>AEAGITGTWYAQLGDTFIVTAGADGALTGTYEAAVGDDDGDDDGDDDGAESRYVLTGRYDSAPATDGSGTALGWTVAWKNNYRNAHSATTWSGQYVGGAEARINTQWLLTSGTTEANAWKSTLVGHDTFTKVKPSAAS[2x];>AEAGITGTWYNQLGSTFIVTAGADGALTGTYESAVGNAESRYVLTGRYDSAPATDGSGTALGWTVAWKNNYRNAHSATTWSGQYVGGAEARINTQWLLTSGTTEANAWKSTLVGHDTFTKVKPSAAS[2x]

The femtomolar affinity of streptavidin/avidin for biotinylated targets, combined with resilience to harsh conditions and an on-rate of ~ 107 M− 1 s− 1, is the basis for biotin's central role as a specific biological “glue” in diverse research methods and biotechnologies. We previously generated streptavidin heterotetramers with exactly one, two, or three functional biotin-binding sites, through purifying tetramers containing defined numbers of non-biotin-binding “Dead” and His6-tagged wild-type subunits. However, tetramers with two functional and two Dead subunits can assemble in three different arrangements. To generate a controlled and stable bridge for bionanotechnology, we demonstrate here a method for the simple isolation of streptavidin variants with precise cis-divalent or 1,3 trans-divalent arrangements.

In the 1,2 arrangement the biotin-binding sites of streptavidin are in a cis configuration as the binding sites both point in the same direction. To isolate cis-divalent streptavidin (1,2 arrangement of biotin-binding subunits), we introduced a series of aspartates into the loop between β-strands 3 and 4 (L3,4) of the Dead subunit. Introduction of the charges in this position means that in the 1,3 and 1,4 arrangements, these charged regions should be far apart, while in the 1,2 arrangement, the charged loops should be apposed. Since L3,4 is important for biotin binding affinity, it was necessary to insert these residues on the Dead subunit, so that the cis-divalent streptavidin could maintain high biotin binding affinity. Overall, the introduction of a series of negative charges into the surface-exposed 3,4-loop of streptavidin allowed the isolation of a second divalent species, cis-divalent. However, one condition obtained using the Morpheus crystal screen yielded the desired asymmetric unit for the cis-divalent streptavidin containing all four subunits. The obtained 1,3 trans-divalent crystal structure was solved at 1.6 Å resolution, and cis-divalent streptavidin was solved at 1.4 Å resolution, with the phases in each case solved using molecular replacement. For the putative cis-divalent sample, the electron density closely fits if chains a/c are Dd and chains b/d are SA, also confirming that the biotin-binding subunits indeed had a cis orientation. Furthermore, while the electron density around L3,4 could be clearly observed in the SA chains b and d of the cis-divalent form, the electron density of L3/4 was poorly defined in Dd chains a and c. The engineered L3,4 of Dd (chains a/c) is expected to be highly flexible, which would lead to weak diffraction in this region.> TSWSDRLQNAADMPANMDKHALKKYRREAYHRVFVNRSLAMEKIKCFGFDMDYTLAVYKSPEYESLGFELTVERLVSIGYPQELLSFAYDSTFPTRGLVFDTLYGNLLKVDAYGNLLVCAHGFNFIRGPETREQYPNKFIQRDDTERFYILNTLFNLPETYLLACLVDFFTNCPRYTSCETGFKDGDLFMSYRSMFQDVRDAVDWVH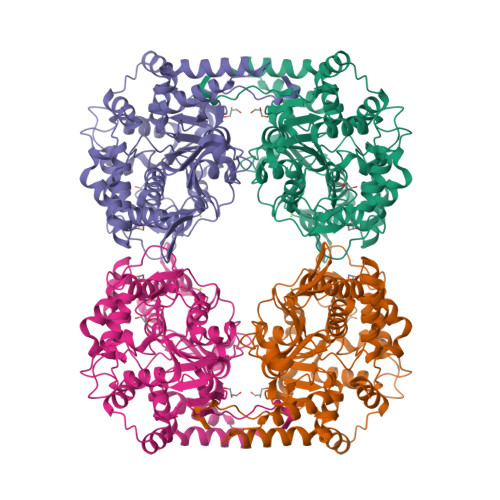YKGSLKEKTVENLEKYVVKDGKLPLLLSRMKEVGKVFLATNSDYKYTDKIMTYLFDFPHGPKPGSSHRPWQSYFDLILVDARKPLFFGEGTVLRQVDTKTGKLKIGTYTGPLQHGIVYSGGSSDTICDLLGAKGKDILYIGDHIFGDILKSKKRQGWRTFLVIPELAQELHVWTDKSSLFEELQSLDIFLAELYKHLDSSSNERPDISSIQRRIKKVTHDMDMCYGMMGSLFRSGSRQTLFASQVMRYADLYAASFINLLYYPFSYLFRAAHVLMPHES> MGSSHHHHHHSSENLYFQGHMASDYLDVVPPEQPNIDDAMSSPTRALGFLYSCYGGVSTDLPSAYLGEINSTTDEYVLPYSWNTDGYWGAYAFNTASSTNQDWLWGTTYQYIGQCYLFLQKLENAGSDIASDAEKEQWRAECQFLVAYYHFATLRRYGPIPITDSYIPMDTPTSEYNGRFHFDYCVDWIANQLDEAAKVLPANRTVTNEWGRATSTIAKAVKARLLLYAASPLWNGSFPYPNWQNENFETPGYGKALVSNTYDKSKWERALAACQEALTLATTSGDRELYDDDEYYSRQSLNLPFVPGVADVEDNKEFLKNVMKMRYAVSTRESEGNKEIIWGLSNQFDFYSRYPLRILKKSDGTWHAGYSGVSPTLYTFEHFYTANGKLPEKDLDFTPSSEWFESAGISSREDIIKLNVGREPRFYAWMAFDGGDY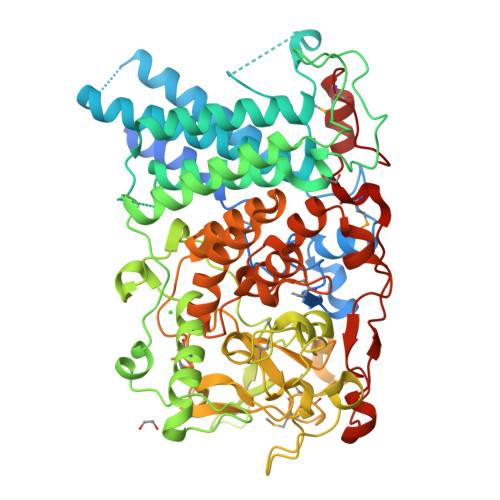GTKFAAGSPLKLEMRNSEMHGYNPSLFNRDHSVTGFLTQKFVDPVTEFYTAGGSTSGTSAPTILFRLAELYLNVAECHAALGNTQEAIDALNPVRERAGIPKLTLADITNNMTIKDWVHNERFVELWNEGHRFFDVRRWAEGAKYFGANKREGLNAEVQSPTFEEFNKRTTVDAPYVWENRMYLNPVFYNEVYKNPQMVQAPGY>GHMKISRETLHQLIENKLCQAGLKREHAATVAEVLVYADARGIHSHGAVRVEYYAERISKGGTNREPEFRLEETGPCSAILHADNAAGQVAAKMGMEHAIKTAQQNGVAVVGISRMGHSGAISYFVQQAARAGFIGISMCQSDPMVVPFGGAEIYYGTNPLAFAAPGEGDEILTFDMATTVQAW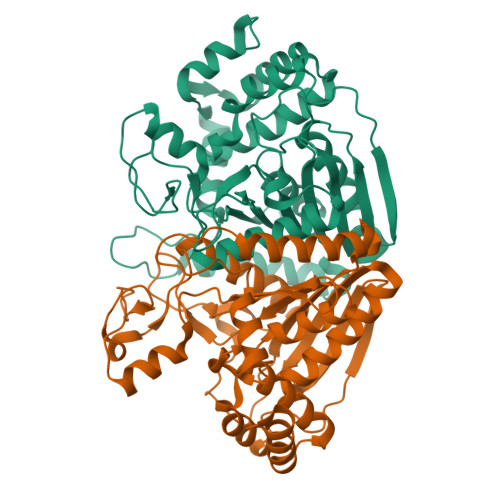GKVLDARSRNMSIPDTWAVDKNGVPTTDPFAVHALLPAAGPKGYGLMMMIDVLSGVLLGLPFGRQVSSMYDDLHAGRNLGQLHIVINPNFFSSSELFRQHLSQTMRELNAITPAPGFNQVYYPGQDQDIKQRKAAVEGIEIVDDIYQYLISDALYNTSYETKNPFAQ[2x]> AVKLSHVEKDFIAFYSTTPHHLSYRDKTGGSYFITRLISCFRKHACSCHLFDIFLKVQQ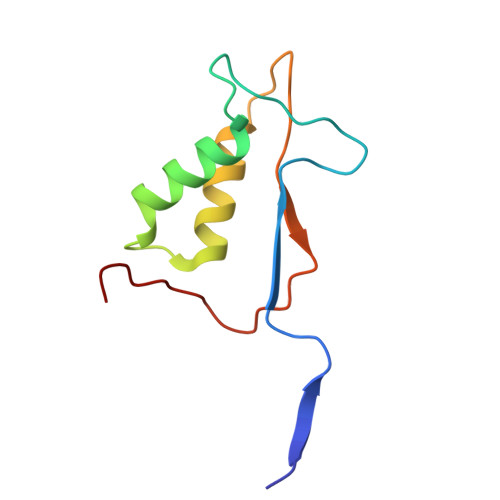SFEKASIHSQMPTIDRATLTRYFYLFPGN Insect Toll receptors perform critical functions in both embryogenesis and innate immunity. Toll receptors are activated by a complementary family of six cytokine-like molecules called Spaetzle (Spz). Three oligomeric states of the receptor were observed at near-atomic resolutions, suggesting that Toll5A is highly dynamic in the presence of Spz1C.

A third particle was observed with a stoichiometry of 3 receptors and 1 ligand. Homodimers of Toll5A at 3.41 Å maximum resolution had 85,810 particles, 2:1 heterodimers of Toll5A bound to Spz1C at 4.23 Å had 40,153 particles, and a 3:1 heterotrimer at 3.74 Å had 42,866 particles. The three Toll5A molecules observed are referred to as chain A (teal), chain B (dark blue) and chain C (powder blue) in superimposable conformations in all three structures (RMSD below 2 Å). The vacated ligand binding site is occupied by another receptor chain in the 3:1 heterotrimer, illustrating the transition between homo- and heterodimerisation. While binding of a first Spz1C ligand shifts the receptor to adopt an asymmetric dimer configuration, the second binding site remains predominantly associated to another receptor chain. The N-terminal region of Toll5A (chain B) deviates by an angle of ~60°, compared to the axis traversing chain C from N- to C-terminus. None of these techniques detected the heterotrimer, which is therefore most likely a side effect of cryo-EM’s capacity of visualising transition intermediates.

>[3x]TSTKRFTCPEESEASNCSCEEFPSKTHFYCPDFNPTLYVDVEDRMRVDFKCYDEPHDFKSLPNLAIGSVKLLTVVDCVLDDDRPILESFKFLEVADVRSFVYNNHENGIRYNAKYFEGMEQLENLTLARGVVSIDRDTFSGFLNLKRLTIEHNKLNLQPGTFEALSNLTYLGLVYNGLNEIQPGLFDGLESLEALSLSYNDIKSLSAGSFNGLSSLRMLNLRVNKIESFDANTFASLKELSRLEITLNPFVSLPRGLFSENKKLKTLILTNNRKLVTLPEELLANLKELTVVNLSHNGVGNLPESLLSGSSGIIELNLGYNRLNSLPEELLSDQPQLQVLNLDHNQLESIPDYFLERNVELQTLYLSHNRLRSLSEKAFTKLKNLKELHLENNQLQTIPQFLFSGTPKLEEIYMQNNQLALHANSFINEELSIADNDNTPFQVLQKLRILHLRNNSISTIFQDWYINNLEMQSLDLSFNKLPGLSYTQLQFQSNITLNLSNNEISQVLLIDDLDLQPYQRINVDLNHNPLNCNCNALKFIQLIQSKAEHGLQFNVDQLRCSEPPNLLDATMDQLQTKDLLCDFESADDCPKDCQCAMRLLDHTVIVNCSGRGLTEFPDLPIPSQLHEDFNALEVHVENNRLTKLPNLTKHNEITQLYARNNSIQNLLPHNIPSKLRIIDLSQNLLKMIDDSTLAQINRSSHLETIRLSQNQWLCDCPASSFLIFVQQNSRLISDMSAIRCHPSGKSLDSITVNELCFEDYTTENLYFQ;>[2x]GSDTANAPFLCESEQLLIHPKEELSRNNSMVWIVNTKDYKQGVRIEKCLKRQLGKPCNFCDADTECKQLFHYRTLVAVDKVTKKPYKEQVLLPSCCKCAKILSTGWSHPQFEK>[4x]CG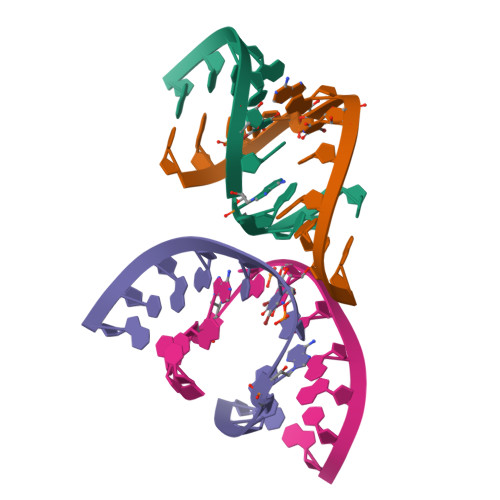CGAAUUAGCG>[2x]SQLAHNLTLSIFDPVANYRAARIICTIGPSTQSVEALKGLIQSGMSVARMNFSHGSHEYHQTTINNVRQAAAELGVNIAIALDTKGPEIRTGQFVG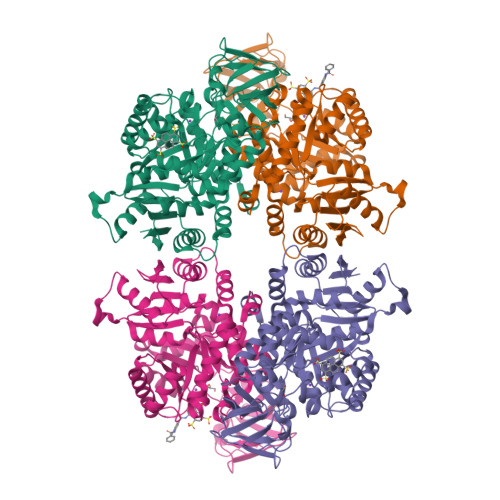GDAVMERGATCYVTTDPAFADKGTKDKFYIDYQNLSKVVRPGNYIYIDDGILILQVQSHEDEQTLECTVTNSHTISDRRGVNLPGCDVDLPAVSAKDRVDLQFGVEQGVDMIFASFIRSAEQVGDVRKALGPKGRDIMIICKIENHQGVQNIDSIIEESDGIMVARGDLGVEIPAEKVVVAQKILISKCNVAGKPVICATQMLESMTYNPRPTRAEVSDVANAVFNGADCVMLSGETAKGKYPNEVVQYMARICLEAQSALNEYVFFNSIKKLQHIPMSADEAVCSSAVNSVYETKAKAMVVLSNTGRSARLVAKYRPNCPIVCVTTRLQTCRQLNITQGVESVFFDADKLGHDEGKEHRVAAGVEFAKSKGYVQTGDYCVVIHADHKVKGYANQTRILLVE> GVGVSTGSYDNQTHYRFLGDGWVEITALATRLVHLNMPKSENYCRIRVHNTTDTSVKGNMAKDDAHEQIWTPWSLVDANAWGVWLQPSDWQYICNTMSQLNLVSLDQEIFNVVLKTVTEQDLGGQAIKIYNADLTACMMVAVDSNNILPYTPAANSMETLGFYPWKPTIASPYRYYFCVDRDLSVTYENQEGTVEHNVMGTPKGMNSQFFTIENTQQITLLRTGDEFATGTYYFDTNPVKLTHTWQTNRQLGQPPLLSTFPEADTDAGTLTAQGSRHGTTQMGVNWVSEAIRTRPAQVGFCQPHNDFEASRAGPFAAPKVPADITQGVDKEANGSVRYSYGKQHGENWASHGPAPERYTWDETSFGSGRDTKDGFIQSAPLVVPPPLNGILTNANPIGTKNDI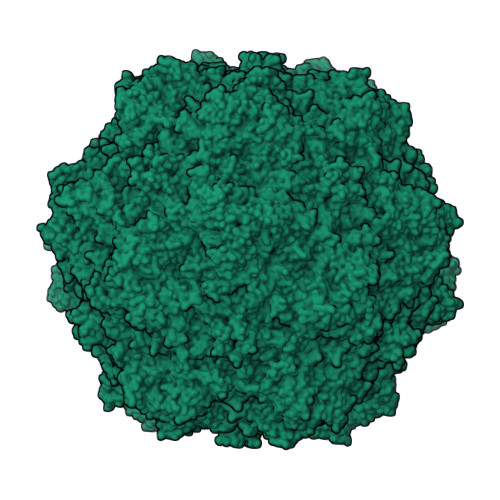HFSNVFNSYGPLTAFSHPSPVYPQGQIWDKELDLEHKPRLHITAPFVCKNNAPGQMLVRLGPNLTDQYDPNGATLSRIVTYGTFFWKGKLTMRAKLRANTTWNPVYQVSAEDNGNSYMSVTKWLPTATGNMQSVPLITRPVARNTY>[8x]EVDPRLYFENRSKFIQDQKDKGINPYPHKFERTISIPEFIEKYKDLGNGEHLEDTILNITGRIMRVSASGQKLRFFDLVGDGEKIQVLANYSFHNHEKGNFAECYDKIRRGDIVGIVGFPGKSKKGELSIFPKETILLSACLHMLPMKYGLKDTEIR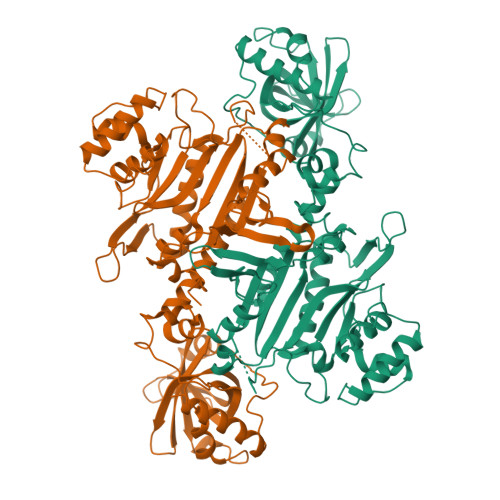YRQRYLDLLINESSRHTFVTRTKIINFLRNFLNERGFFEVETPMMNLIAGGANARPFITHHNDLDLDLYLRIATELPLKMLIVGGIDKVYEIGKVFRNEGIDNTHNPEFTSCEFYWAYADYNDLIKWSEDFFSQLVYHLFGTYKISYNKDGPENQPIEIDFTPPYPKVSIVEEIEKVTNTILEQPFDSNETIEKMINIIKEHKIELPNPPTAAKLLDQLASHFIENKYNDKPFFIVEHPQIMSPLAKYHRTKPGLTERLEMFICGKEVLNAYTELNDPFKQKECFKLQQKDREKGDTEAAQLDSAFCTSLEYGLPPTGGLGLGIDRITMFLTNKNSIKDVILFPTMRPAN> MILPPIPTPFDREGRLDEEAFRELAQALEPLVDGLLVYGSNGEGVHLTPEERARGLRALRPRKPFLVGLMEETLPQAEGALLEAKAAGAMALLATPPRYYHGSLGAGLLRYYEALAEKMPLFLYHVPQNTKVDLPLEAVEALAPHPNVLGIKDSSGDLSRIAFYQARLQEFRVYTGHAPTFLGALALGAEGGILAAA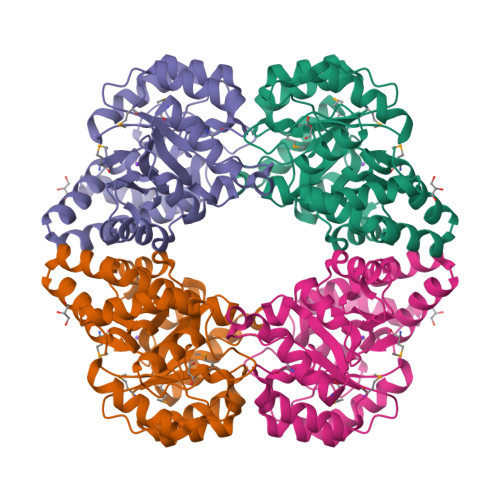NLAPRAYRALLDHFREGRLAEAQELQKKLFPLGDLLAKGGVPLLKQALRHLGLPAGYPRPPYPAESPLWERFLPVLEGLKEEGWVL> SMLTFREVVSPQEFKQGEDAEVVCRVSSSPAPAVSWLYHNEEVTTISDNRFAMLANNNLQILNINKSDEGIYRCEGRVEARGEIDFRDIIVIVNVPPAISMPQKSFNATAERGEEMTFSCRASGSPEPAISWFRNGKLIEENEKYILKGSNTELTVRNIINSDGGPYVCRATNKA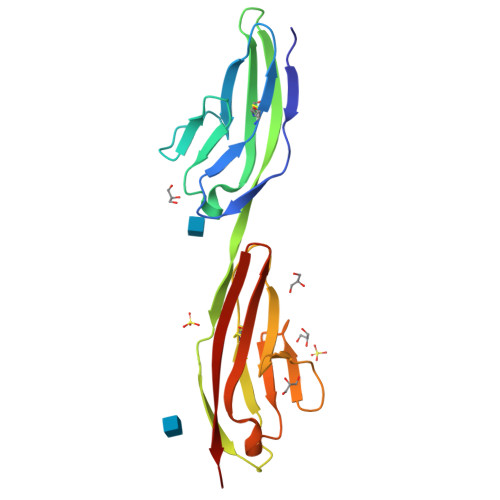GEDEKQAFLQVFVQ> MESKRNKPG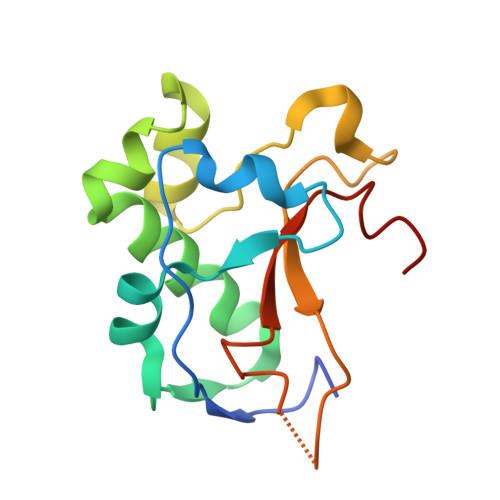KATGKGKPVGDKWLDDAGKDSGAPIPDRIADKLRDKEFKNFDDFRKKFWEEVSKDPDLAKQFKRSNRKRIQQGYAPFAPQKDQVGGRTTFELHHDKPISQDGGVYDMNNIRVTTPKRAIDIHRGK> FWF;> FY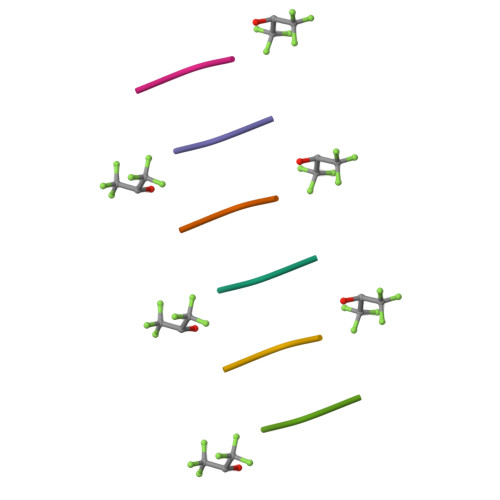F>[2x]MKFAEHLSAHITPEWRKQYIQYEAFKDMLYSAQDQAPSVEVTDEDTVKRYFAKFEEKFFQTCEKELAKINTFYSEKLAEAQRRFATLQNELQSSLDAQKESTGVTTLRQRRKPVFHLSHEERVQHRNIKDLKLAFSEFYLSLILLQNYQNLNFTGFRKILKKHDKILETSRGADWRVAHVEVAPFYTCKKINQLISETEAVVTNELEDGDRQKAMKRLRVPPLGAAQPAPAWTTFRVGLFCGIFIVLNITLVLAAVFKLETDRSIWPLIRIYRGGFLLIEFLFLLGINTYGWRQAGVNHVLIFELNPRSNLSHQHLFEIAGFLGILWCLSLLACFFAPISVIPTYVYPLALYGFMVFFLINPTKTFYYKSRFWLLKLLFRVFT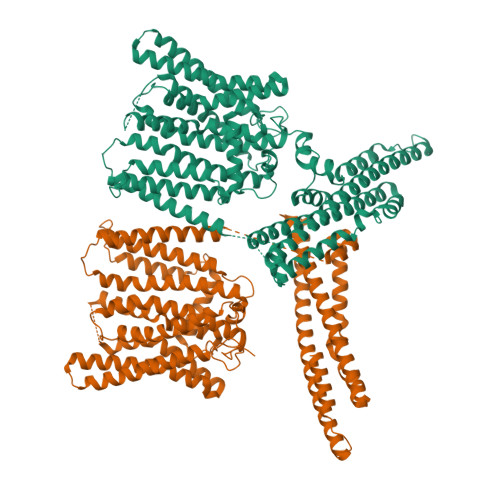APFHKVGFADFWLADQLNSLSVILMDLEYMICFYSLELKWDESKGLLPNNSEESGICHKYTYGVRAIVQCIPAWLRFIQCLRRYRDTKRAFPHLVNAGKYSTTFFMVTFAALYSTHKERGHSDTMVFFYLWIVFYIISSCYTLIWDLKMDWGLFDKNAGENTFLREEIVYPQKAYYYCAIIEDVILRFAWTIQISITSTTLLPHSGDIIATVFAPLEVFRRFVWNFFRLENEHLNNCGEFRAVRDISVAPLNADDQTLLEQMMDQDDGVRNRQKNRSWKYNQSISLRRPRLASQSKARDTKVLIEDTDDEANTENLYFQGHHHHHHHHSGAAAWSHPQFEK> MISTTISGKRPIEQVDDELLSLTAQQENEEQQQQRKRRRHQFAPMTQFNSNTLDEDSGFRSSSDVATADQDNFLEESPSGYIKKVILRNFMCHEHFELELGSRLNFIVGNNGSGKSAILTAITIGLGAKASETNRGSSLKDLIREGCYSAKIILHLDNSKYGAYQQGIFGNEIIVERIIKRDGPASFSLRSENGKEISNKKKDIQTVVDYFSVPVSNPMCFLSQDAARSFLTASTSQDKYSHFMKGTLLQEITENLLYASAIHDSAQENMALHLENLKSLKAEYEDAKKLLRELNQTSDLNERKMLLQAKSLWIDVAHNTDACKNLENEISGIQQKVDEVTEKIRNRQEKIERYTSDGTTIEAQIDAKVIYVNEKDSEHQNARELLRDVKSRFEKEKSNQAEAQSNIDQGRKKVDALNKTIAHLEEELTKEMGGDKDQMRQELEQLEKANEKLREVNNSLVVSLQDVKNEERDIQHERESELRTISRSIQNKKVELQNIAKGNDTFLMNFDRNMDRLLRTIEQRKNEFETPAIGPLGSLVTIRKGFEKWTRSIQRAISSSLNAFVVSNPKDNRLFRDIMRSCGIRSNIPIVTYCLSQFDYSKGRAHGNYPTIVDALEFSKPEIECLFVDLSRIERIVLIEDKNEARNFLQRNPVNVNMALSLRDRRSGFQLSGGYRLDTVTYQDKIRLKVNSSSDNGTQYLKDLIEQETKELQNIRDRYEEKLSEVRSRLKEIDGRLKSTKNEMRKTNFRMTELKMNVGKVVDTGILNSKINERKNQEQAIASYEAAKEELGLKIEQIAQEAQPIKEQYDSTKLALVEAQDELQQLKEDINSRQSKIQKYKDDTIYYEDKKKVYLENIKKIEVNVAALKEGIQRQIQNACAFCSKERIENVDLPDTQEEIKRELDKVSRMIQKAEKSLGLSQEEVIALFEKCRNKYKEGQKKYMEIDEALNRLHNSLKARDQNYKNAEK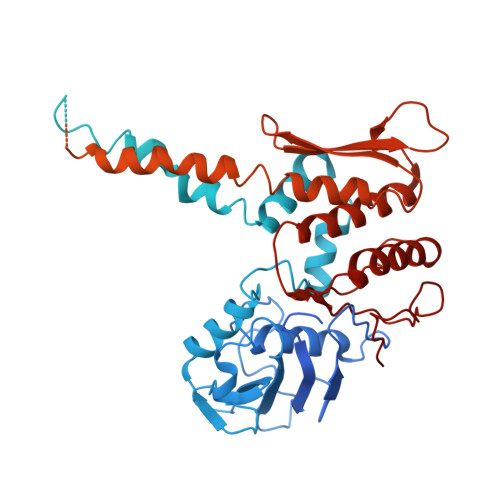GTCFDADMDFRASLKVRKFSGNLSFIKDTKSLEIYILTTNDEKARNVDTLSGGEKSFSQMALLLATWKPMRSRIIALDQFDVFMDQVNRKIGTTLIVKKLKDIARTQTIIITPQDIGKIADIDSSGVSIHRMRDPERQNNSNFYN> AA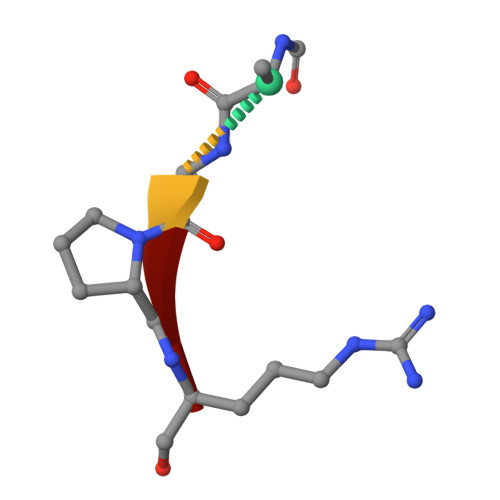PR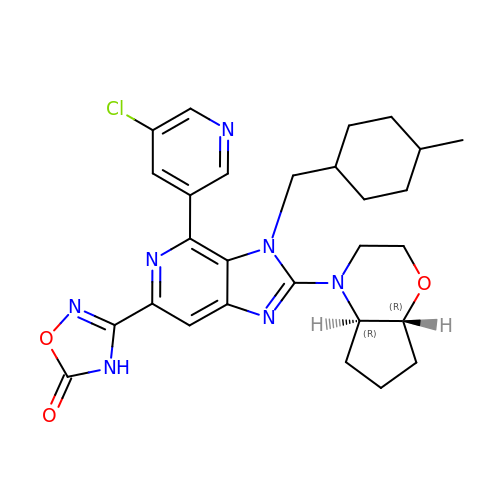3-[4-(5-chloropyridin-3-yl)-2-[(4aR,7aR)-hexahydrocyclopenta[b][1,4]oxazin-4(4aH)-yl]-3-{[(1r,4R)-4-methylcyclohexyl]methyl}-3H-imidazo[4,5-c]pyridin-6-yl]-1,2,4-oxadiazol-5(4H)-one | C28 H32 Cl N7 O3 | FDBWTMMKIZGUEZ-IEGYKGNPSA-N>MNLIPTVIETTNRGERAYDIYSRLLKDRIIMLGSQIDDNVANSIVSQLLFLQAQDSEKDIYLYINSPGGSVTAGFAIYDTIQHIKPDVQTICIGMAASMGSFLLAAGAKGKRFALPNAEVMIHQPLGG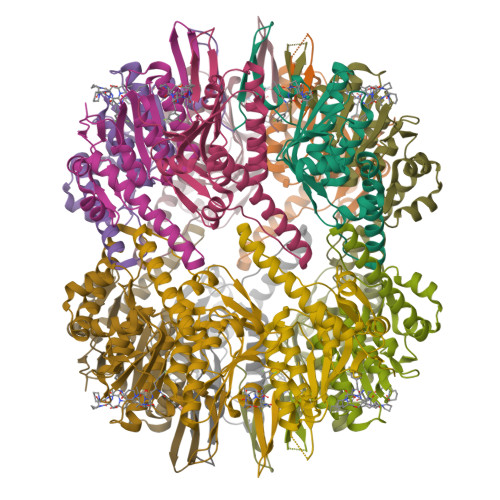AQGQATEIEIAANHILKTREKLNRILSERTGQSIEKIQKDTDRDNFLTAEEAKEYGLIDEVMVPETKWSHPQFEK[7x]> MSTPARRRLMRDFKRMKEDAPPGVSASPLPDNVMVWNAMIIGPADTPYEDGTFRLLLEFDEEYPNKPPHVKFLSEMFHPNVYANGEICLDILQNRWTPTYDVASILTSIQSLFNDPNPASPANVEAAT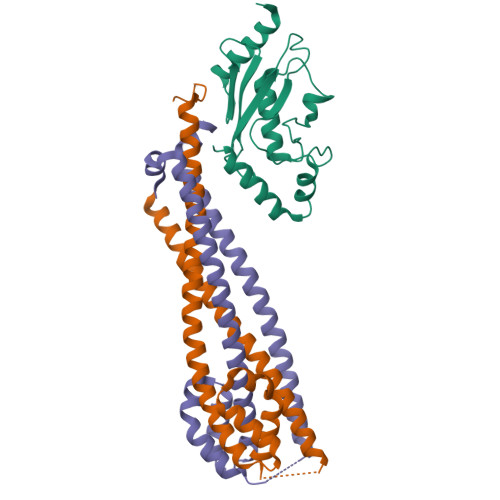LFKDHKSQYVKRVKETVEKSWE;>[2x]MTAEPATKKIKLELSDPSEPLTQSDVIAFQKEALFRCINRRRVDFEALRKQYELSRRECIDVSRKLANIMALIVTLARFIETFCTDANEKQLCREIAQGDETLIVQRSDSFMKLLTKYGKPNTTDSNTNSNASDHIQELTTELKNLRKSKEELFYENSQLTEEISALKEYYTNIIRKYDRDESFTIKRVFKEDKTDAVKELREDEKESNENN>MRLSYEALEWRTPIENSTEPVSLPPPPPFFGQERAREALELAIRGGFHAYLVGPPSLGKHEALLAYLSTQSVETPPDLLYVPLSERKVAVLTLPSGQEIHLAEAVEGLLLEVNRLDELFRQGSFLREKTQLEARFKEAREQQLEALRREAQEAGFALSTNGERLELTGPGPVPAELSARLEEVTLGSLAASAELEVALRRLRRDWALHYLNNRFEPLFQRFPQARAYLEALRARLARYAETGEPLDPAQWRPNLLTSSSSGTPPPIVYEPYATAPRLFGRLDYLVDRGVWSTNVSLIRPGAVHRAQGGYLILDALSLKREGTWEAFKRALRNGQVEPVTEPQAPAGLEVEPFPIQMQVILVGTPEAFEGLEEDPAFSELFRIRAEFSPTLPASPENCTALGGWLLAQGFQLTQGGLTRLYDEARRMAEQRDRMDARLVEIRALAEEAAVLGGGLLTAESVEQAIAAREHRSFLSEEEFLRAVQEGVIRLRTTGRAVGEVNSLVVVEAAPYWGRPARLTARAAPGRDH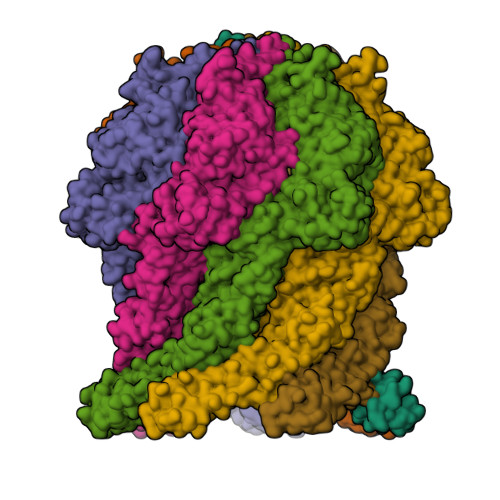LISIDREAGLGGQIFHKAVLTLAGYLRSRYIEHGSLPVTISLAFEQNYVSIEGDAAGLAELVAALSAIGNLPLRQDLAVTGAVDQTGKVLAVGAINAKVEGFFRVCKALGLSGTQGVILPEANLANLTLRAEVLEAVRAGQFHIYAVETAEQALEILAGARMEGFRGLQEKIRAGLEAFARLEEGHDKEDREKLAAALEHHHHHH[7x]>[2x]AEAGITGTWYNQLGSTFIVTAG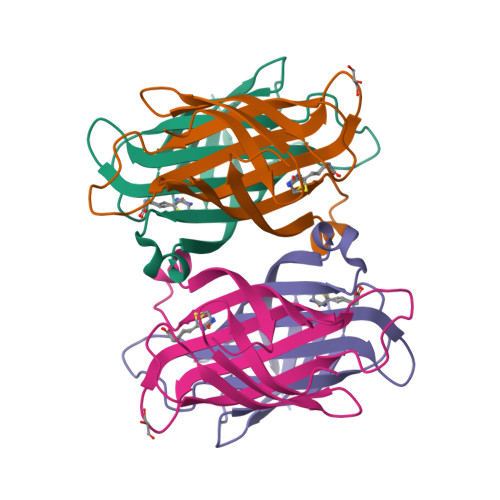ADGALTGTYESAVGNAESRYVLTGRYDSAPATDGSGTALGWTVAWKNNYRNAHSATTWSGQYVGGAEARINTQWLLTSGTTEANAWKSTLVGHDTFTKVKPSAAS>[2x]GGADQKGPVFLKEPTNRIDFSNSTGAEIECKASGNPMPEIIWIRSDGTAVGDVPGLRQISSDGKLVFPPFRAEDYRQEVHAQVYACLARNQFGSIISRDVHVRAVVNQ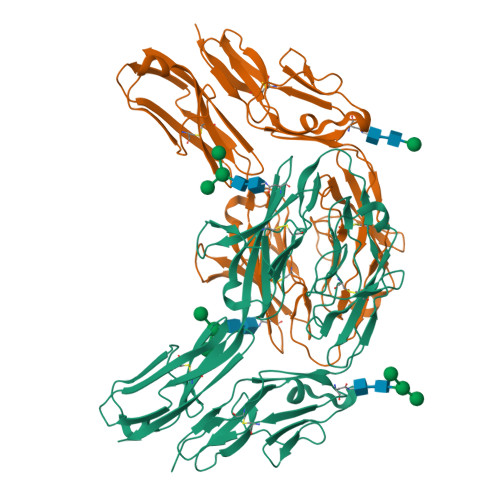FYGADILMEYVIRGNAAVLKCSIPSFVADFVRVESWIDEEGTELRPSENYDGKYLVLPSGELHIREVGPEDGYKSYQCRTKHRLTGETRLSATKGRLVITEPVGSKAPTFATASKISSLLGSSSSDIVLLCQAQAFPVPYTRWYKFIEGTTRKQAVVLNDRVKQVSGTLIIKDAVVEDSGKYLCVVNNSVGGESVETVLTVTAPLSAKIDPPTQTVDFGRPAVFTCQYTGNPIKTVSWMKDGKAIGHSEPVLRIESVKKEDKGMYQCFVRNDQESAEASAELKLGG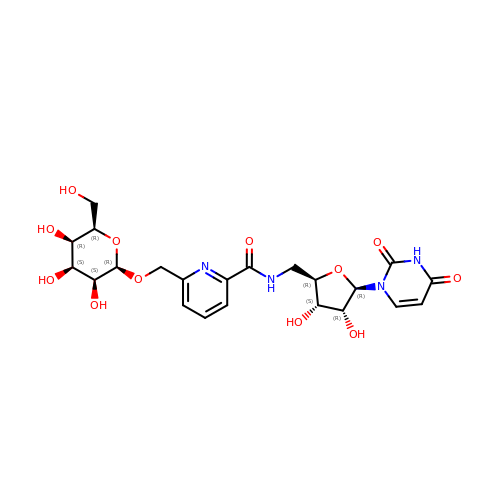6-(1-beta-D-Galactopyranosyloxymethyl)-N-(5'-deoxyluridine-5'-yl)picolinamide | C22 H28 N4 O12 | KPOTWZYLDCHCIG-GBMKPDNQSA-N>ETQELASKRVDIQNKRFYLDVKQNAKGRFLKIAEVGAGGNKSRLTLSMSVAVEFRDYLGDFIEHYAQLGPSQPPDLAQAQDEPRRALKSEFLVRENRKYYMDLKENQRGRFLRIRQTVNRGPGLGSTQGQTIALPAQGLIEFRDALAKLIDDYGVE[4x]

Mutations in the human PURA gene cause the neurodevelopmental PURA syndrome. Based on the crystal structures of PURA from Drosophila melanogaster (dmPURA), three conserved sequence regions termed PUR repeats I, II, and III were identified to fold into globular domains. Whereas PUR repeat I and II assemble into an N-terminal PUR domain via intramolecular interactions, two C-terminal PUR repeats III from different molecules interact with each other and thus mediate dimerization of PURA. All these PUR domains belong to the class of the PC4-like protein family, which mainly bind single-stranded nucleic acids and can unwind double-stranded DNA and RNA.

For a better understanding of the structural impact of genetic variations in the N-terminal PUR domain (hsPURA I–II), we determined its structure (fragments E57–E212) by X-ray crystallography. The N-terminal PUR domain resembles the previously published PURA structure from D. melanogaster (dmPURA I–II WT) with an average r.m.s.d. of 1.2 Å. However, in contrast to this invertebrate structure, we observed for hsPURA I–II that the four molecules within its asymmetric unit of the crystal lattice showed marked differences in its loop regions and in particular at the edges of the β-sheets. This suggested greater structural flexibility than average domain folds and most likely than its D. melanogaster ortholog. Already the different molecules of wild-type hsPURA I–II in the crystal unit cell revealed considerable conformational freedom, not only for narrow movements of the loops but also in the folding of the β-strands. For instance, in some of the molecules in the asymmetric unit of the wild-type hsPURA I–II crystal, β4 and β8 strands formed bulges. From all the areas of the structure, the β-ridge appears to be structurally the most divergent part. Determination of the crystal structure of hsPURA I–II revealed larger flexible regions than the previously reported invertebrate structures, with considerable differences in the four molecules of hsPURA I–II in the asymmetric unit of the crystals. These observations provide clear evidence that in particular strands β4 and β8 of the N-terminal PUR domain are dynamic and can adopt considerable local differences within the β-sheet.>GHMGKPDISAKDLRNI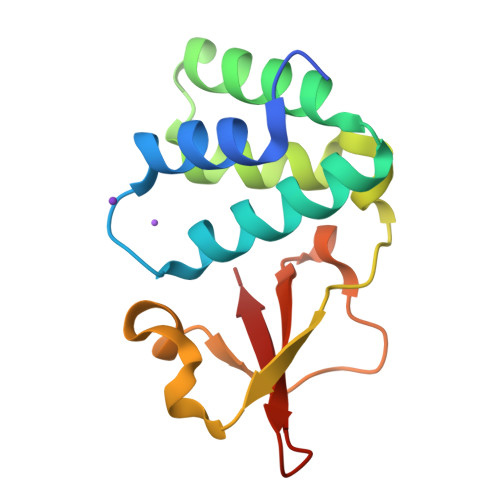MYDHLPGFGTAFHQLVQVICKLGKDSNSLDIIHAEFQASLAEGDSPQCALIQITKRVPIFQDAAPPVIHIRSRGDIPRACQKSLAPVPPSPAIDAGWVCVFQLQDGKTLGLKI[4x]> SSGKV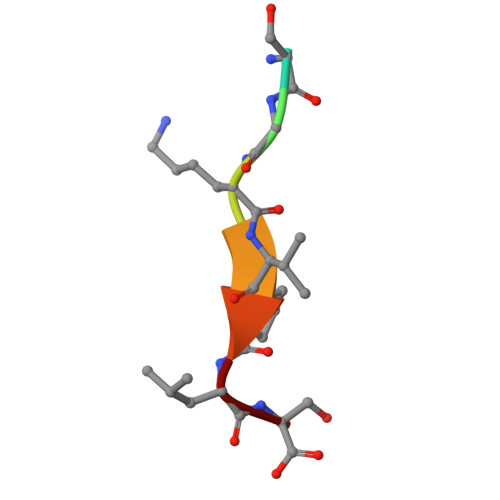PLS>[6x]XARPLEQAVAAIVCTFQEYAGRCGDKYKLAQA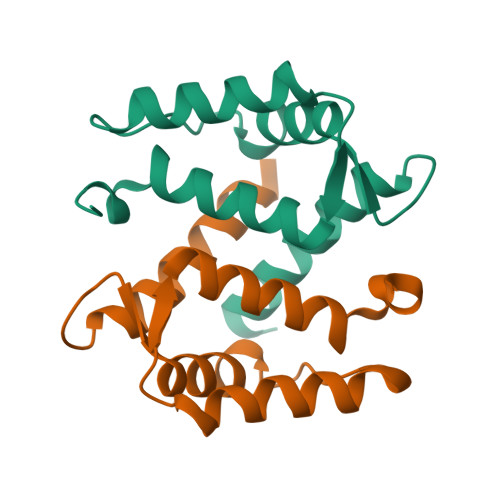ELKELLQKELATWTPTEFRECDYNKFMSVLDTNKDAEVDFVEYVRSLACLCLYCHEYFKDCPSEPPCSQ> MAKQYDSVECPFCDEVSKYEKLAKIGQGTFGEVFKARHRKTGQKVALKKVLMENEKEGFPITALREIKILQLLKHENVVNLIEICRTKASPYNRCKGSIYLVFDFCEHDLAGLLSNVLVKFTLSEIKRVM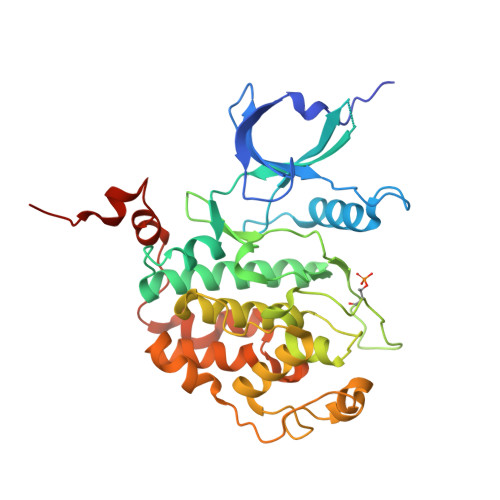QMLLNGLYYIHRNKILHRDMKAANVLITRDGVLKLADFGLARAFSLAKNSQPNRYTNRVVTLWYRPPELLLGERDYGPPIDLWGAGCIMAEMWTRSPIMQGNTEQHQLALISQLCGSITPEVWPNVDNYELYEKLELVKGQKRKVKDRLKAYVRDPYALDLIDKLLVLDPAQRIDSDDALNHDFFWSDPMPSDLKGMLSTHLTSMFEYLAPPRRKHHHHHH N-[2-OXO-3-((E)-PHENYL{[4-(PIPERIDIN-1-YLMETHYL)PHENYL]IMINO}METHYL)-2,6-DIHYDRO-1H-INDOL-5-YL]ETHANESULFONAMIDE | C29 H32 N4 O3 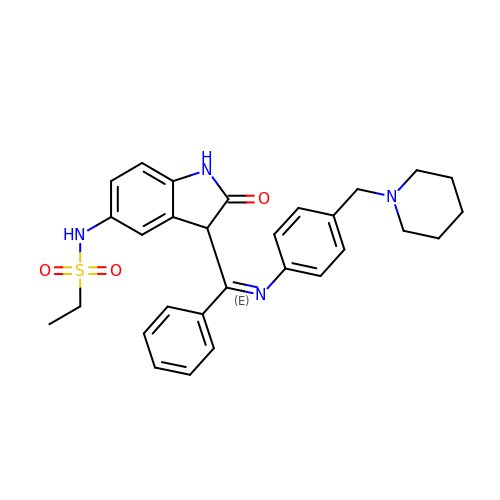S | SGZZQKMOFHIDKW-MCKMWFOCSA-N>[2x]MSDEEILEKLRIIVSVGDPKKKYTRFEKIGQGASGTVYTAMDVATGQEVAIRQMNLQQQPKKELIINEILVMRENKNPNIVNYLDSYLVGDELWVVMEYLAGGSLTDVVTETCMDEGQIA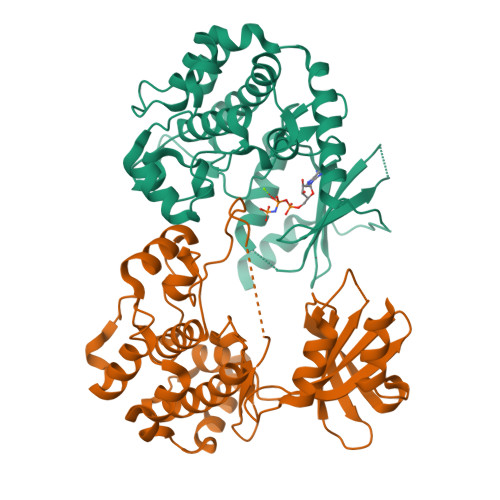AVCRECLQALEFLHSNQVIHRNIKSDNILLGMDGSVKLTDFGFCAQITPEQSKRSTMVGTPYWMAPEVVTRKAYGPKVDIWSLGIMAIEMIEGEPPYLNENPLRALYLIATNGTPELQNPEKLSAIFRDFLNRCLEMDVEKRGSAKELIQHQFLKIAKPLSSLTPLIAAAKEATKNNHLEHHHHHH>[4x]MPLP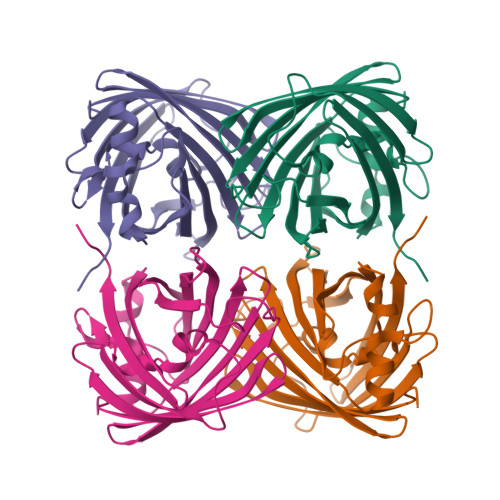KTHELHIFGSFNGVEFDMVGRGIGNPNEGSEELNAKFTKGPLKFSPYILVPHLXYYQYLPFPDGMSPFQAAMHDGSGYQVHRTIQYEDGASVTAHYRYTYEGSHIKGEFQVIGTGFPPDGPVMTNKLTAMDWSVTKMLYPNDKTILSTADCSYTTTAGKRYQSKMRENNTFAKPMAADILQKQPMFVFRKSELQHSKTELTFKEWQKAFTDVMSGGSHHHHHH> MGNKQVKAPEARNSPRASLIPDATHLGPQFCKSCWAENKGLVECNNHYLCLNCLTLLLGVSSRCPICKMPLPTR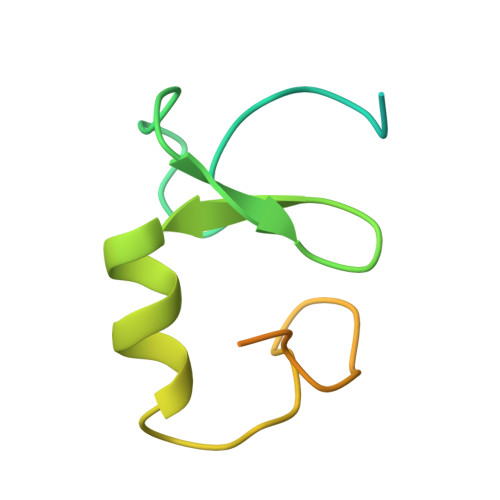LRPSAAPTAPPAEAGDNTRPPPYSP>GSMASAPLRVYVQCNPLLDVSAHVSDEFLVKYGLERGTAILLSERQKGIFDDIEKMPNVRYVPGGSGLNVARVAQWMQQAYKGKFVTYVGCIADDRYGKVLKEAAEHEGIVMAVEHTTKAGSGACAVCITGKERTLVADLGAANHLSSEHM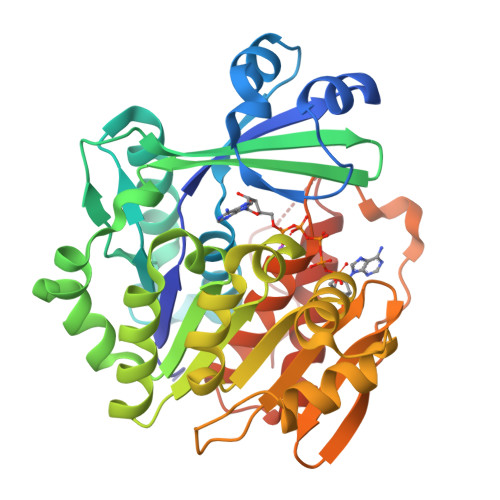RSPAVVRAMDESRIFYFSGFTLTVDVNHVLQACRKAREVDGLFMINLSAPFIMQFFSAQLGEVLPYTDIIVANRHEAKEFANMMKWDTDCVEEIARRAVSEVPYTGTKGRVVVFTRDIESTVLATKDGVETVPVPQLDQDKVIDMNGAGDAFMGGFLSAYAVGKDLRRCCETGHYTAQEVIQRDGCSFPEKPSFSP[2x]>GSHMRSRRVDVMDVMNRLILAMDLMNRDDALRVTGE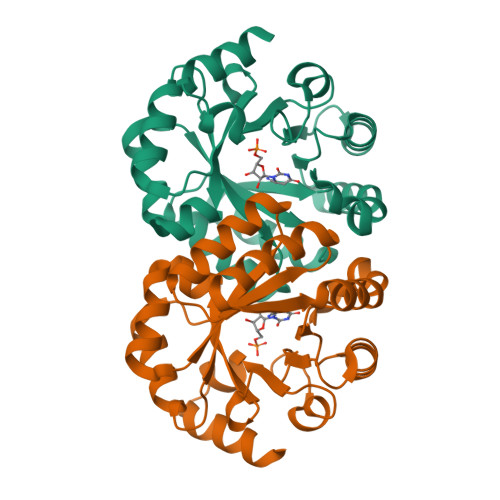VREYIDTVKIGYPLVLSEGMDIIAEFRKRFGCRIIAAFAVADIPETNEKICRATFKAGADAIIVHGFPGADSVRACLNVAEEMGREVFLLTEMSHPGAEMFIQGAADEIARMGVDLGVKNYVGPSTRPERLSRLREIIGQDSFLISPGVGAQGGDPGETLRFADAIIVGRSIYLADNPAAAAAGIIESIKDLRIPEDPAANKARKEAELAAATAEQ[2x]> MPASTYRLQISAEFTLFDAARIVPYLHRLGADWLYLSPLLESEPGSSHGYDVVDHSRVDAARGGPEGLAELSRAAHERGMGVVVDIVPNHVGVATPKANRWWWDVLARGQRSEYADYFDIDWEFGGGRLRLPVLGDGPDELDALRVDGDELVYYEHRFPIAEGTGGGTPREVHDRQHYELMSWRRADHDLNYRRFFAVNTLAAVRVEDPRVFDDTHREIGRWIAEGLVDGLRVDHPDGLRAPGDYLRRLAELAQGRPIWVEKIIEGDERMPPQWPIAGTTGYDALAGIDRVLVDPAGEHPLTQIVDEAAGSPRRWAELVPERKRAVARGILNSEIRRVARELGEVAGDVEDALVEIAAALSVYRSYLPFGREHLDEAVAAAQAAAPQLEADLAAVGAALADPGNPAALRFQQTSGMIMAKGVEDNAFYRYPRLTSLTEVGGDPSLFAIDAAAFHAAQRDRAARLPESMTTLTTHDTKRSEDTRARITALAEAPERWRRFLTEVGGLIGTGDRVLENLIWQAIVGAWPASRERLEAYALKAAREAGESTDWIDGDPAFEERLTRLV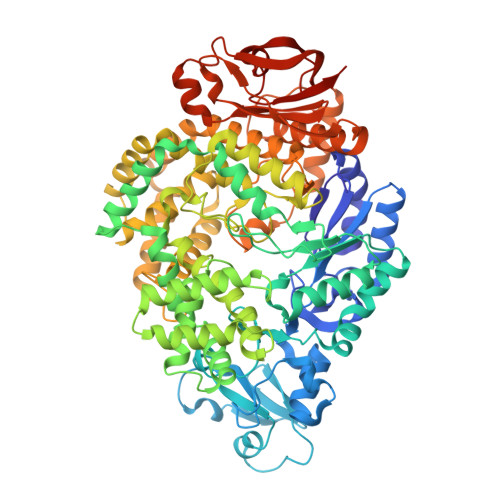TVAVEEPLVHELLERLVDELTAAGYSNGLAAKLLQLLAPGTPDVYQGTERWDRSLVDPDNRRPVDFAAASELLDRLDGGWRPPVDETGAVKTLVVSRALRLRRDRPELFTAYHPVTARGAQAEHLIGFDRGGAIALATRLPLGLAAAGGWGDTVVDVGERSLRDELTGREARGAARVAELFADYPVALLVETKLAAALEHHHHHH> ARVAVLISGTGSNLQALIDSTREPNSSAQIDIVISNKAAVAGLDKAERAGIPTRVINHKLYKNRVEFDSAIDLVLEEFSIDIVCLAGFMRILSGPFVQKWNGKMLNIHPSLLPSFKGSNAHEQALETGVTVTGCTVHFVAEDVDAGQIILQEAVPVKRGD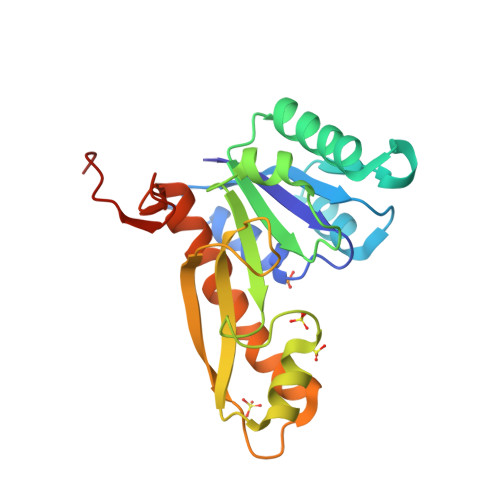TVATLSERVKLAEHKIFPAALQLVASGTVQLGENGKICWVKEEHHHHHH>[3x]GPGYQDPMGVVEEAHNVKVIGSGEATIVLGHGFGTDQSVWKHLVPHLVDDYRVVLYDNMGAGTTNPDYFDFDRYSNLEGYSFDLIAILEDLKIESCIFVGHSVSAMIGVLASLNRPDLFSKIVMISASPRYVNDVDYQGGFEQEDLNQLFEAIRSNYKAWCLGFAPLAVGGDMDSIAVQEFSRTLFNMR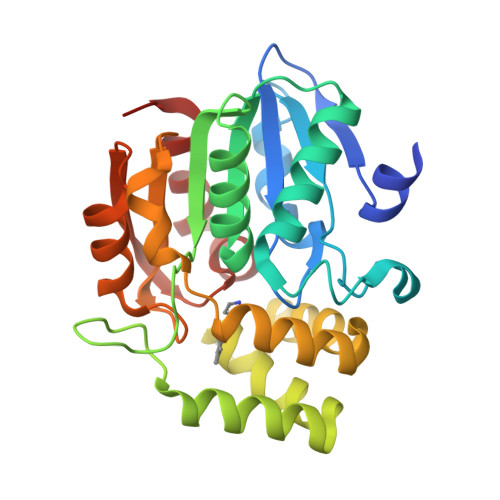PDIALSVGQTIFQSDMRQILPFVTVPCHILQSVKDLAVPVVVSEYLHANLGCESVVEVIPSDGHLPQLSSPDSVIPVILRHIRNDIAM> KTNLANEDEAYEAIFGGEFGSLEIGSYIGGDEGGGSGGGSGGGSADQLEMVTELLGGDMVNQSFICDPDDETFIG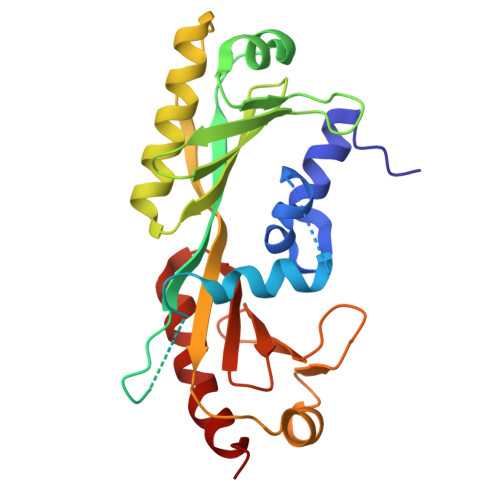GGSGGGSGGGSMSGIVPTLQNIVATVTLGCRLDLKTVALHARNAEYNPKRFAAVIMRIREPKTTALIFASGKMVVTGAKSEDDSKLASRKYARIIQKIGFAAKFTDFKIQNIVGSCDVKFPIRLEGLAFSHGTFSSYEPELFPGLIYRMVKPKIVLLIFVSGKIVLTGAKQREEIYQAFEAIYPVLSEFRKM5-[(2E,4aR,7aR)-6-(5-fluoro-4-methoxy-6-methylpyrimidin-2-yl)-2-imino-3-methyl-4-oxooctahydro-7aH-pyrrolo[3,4-d]pyrimidin-7a-yl]thiophene-2-carbonitrile | C18 H18 F N7 O2 S | 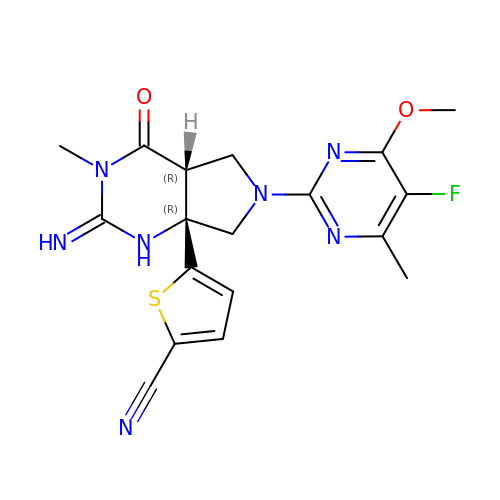ZPAVWCJTQRQRQL-VOJFVSQTSA-N>SFTMSGGFELQPRDGGPRVALAPGETVIGRGPLLGITDKRVSRRHAILEVAGGQLRIKPIHTNPCFYQSSEKSQLLPLKPNLWCYLNPGDSFSLLV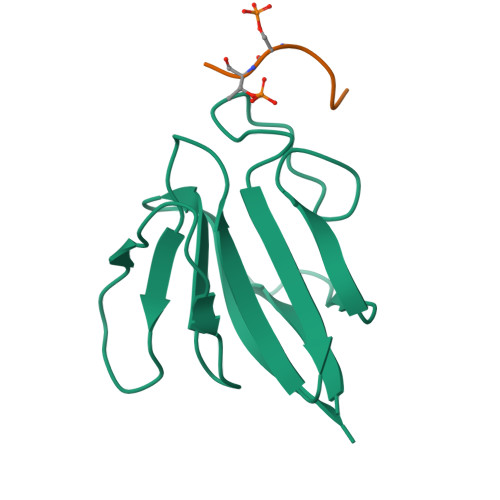DKYIFRILSIPS[4x];>PYAGSTDEN[4x]> SSCKRHPLYVDFSDVGWNDWIVAPPGYHAFYCHGECPFPPADHLNSTNHAIVQTLVNSVNSKIPKAC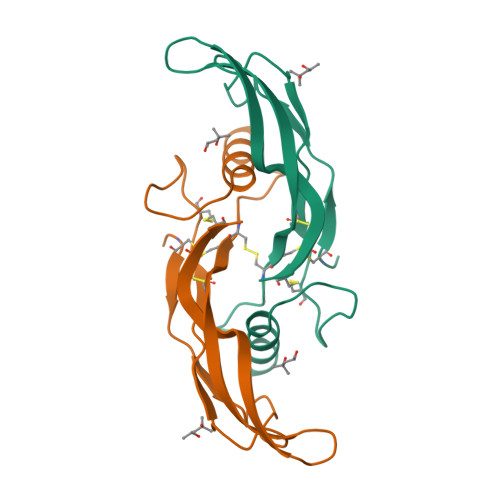CVPTELSAISMLYLDENEKVVLKNYQDMVVEGCGCR> MKRILLVLLTLVFLGAIACQRKEENKTEMVKLKRM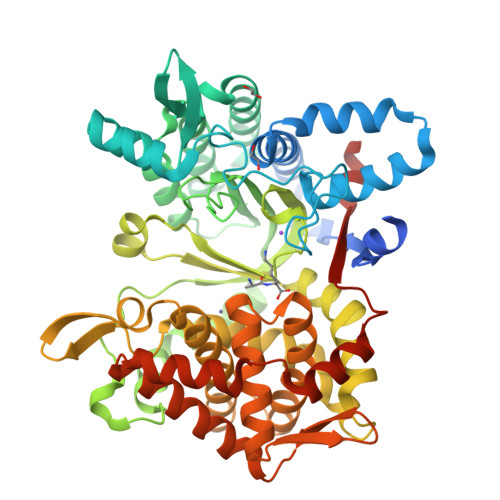IAQFAPTEIKYDHSLLDERKQKVVENLYRAAKIMDEIFLDQVYSKNFEIREQLRASSDPLDQLRLEYFTIMFGPFDRLNHDKPFIGNTPKPKGANFYPPDMTREEFENWLKAHPEDEAAFTSEFTVIRRQDGKLVAIPYSEYYKEYLTRAADYLKKAAEFADNPSLKKYLQLRAEAFLNNDYYESDLAWMDLNDHTIEVVIGPYEVYEDKLFNYKAAFEAFITLRDPVESAKLKKFVGYLDEMEKNLPIPDAYKNFNRGSESPMVVVQEVFSAGDTKAGVQTLAFNLPNDERVREAKGSKKVMLKNIHEAKFDKLLKPIAEKVLFAEQLPLVTFEGFFNHTLMHEISHGLGPGKIVLNGRQTEVKKELKETYSSIEECKADVLGMYNNLFMIEKGVYPPEFEKQIYVTFLAGIFRTIRFGINEAHGAGNAVIFNYLLEKGAYQFDPAAHRVKVNFEKIKDGVRDLANKVLTIQAQGDYMAAKNLLETYAVESEPIMIMRARLQELPVDIKPIFQIEKELGNSNLEHHHHHH>[2x]MTHLFEGVGVALTTPFTNNKVNIEALKTHVNFLLENNAQAIIVNGTTAESP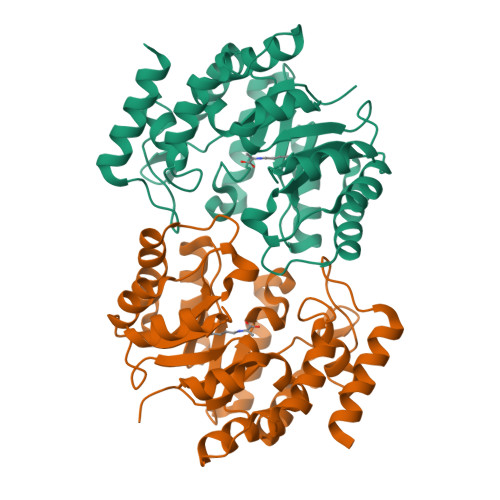TLTTDEKERILKTVIDLVDKRVPVIAGTGTNDTEKSIQASIQAKALGADAIMLITPYYNKTNQRGLVKHFEAIADAVKLPVVLYNVPSRTNMTIEPETVEILSQHPYIVALKDATNDFEYLEEVKKRIDTNSFALYSGNDDNVVEYYQRGGQGVISVIANVIPKEFQALYDAQQSGLDIQDQFKPIGTLLSALSVDINPIPIKALTSYLGFGNYELRLPLVSLEDTDTKVLRETYDTFKAGENE> MKVLYFAEIKDILQKAQEDIVLEQALTVQQFEDLLFERYPQINNKKF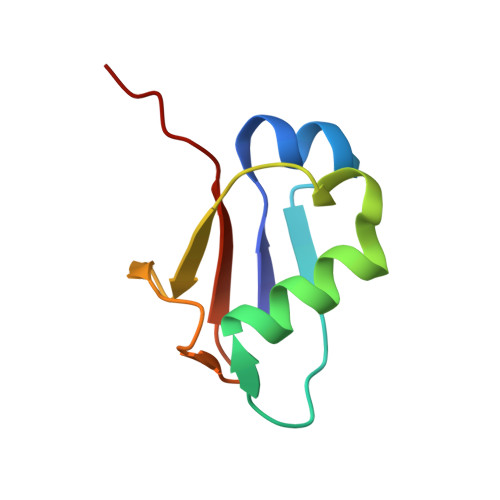QVAVNEEFVQKSDFIQPNDTVALIPPVSGG> FIFLALLGAAVAFPVDDDDKIVGGYTCGANTVPYQVSLNSGYHFCGGSLINSQWVVSAAHCYKSGIQVRLGEDNINVVEGNEQFISASKSIVHPSYNSNTLNNDIMLIKLKSAASLNSRVASISLPTSCASAGTQCLISGWGNTKSSGTSYPDVLKCLKAPILSDSSCKSAYPGQITSNMFCAGYLEGGKDSCQGDAGGPVVCSGKLQGIVSW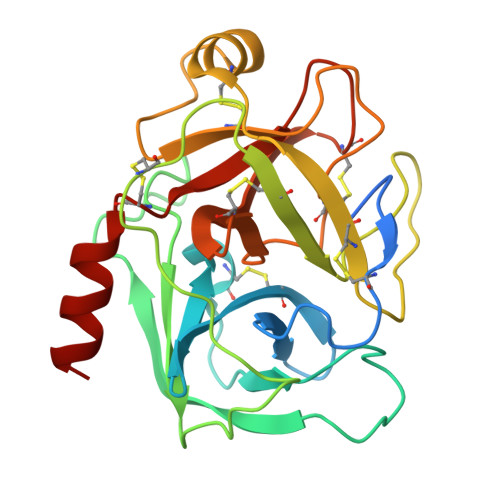GSGCAQKNKPGVYTKVCNYVSWIKQTIASN>[3x]HHHHHHG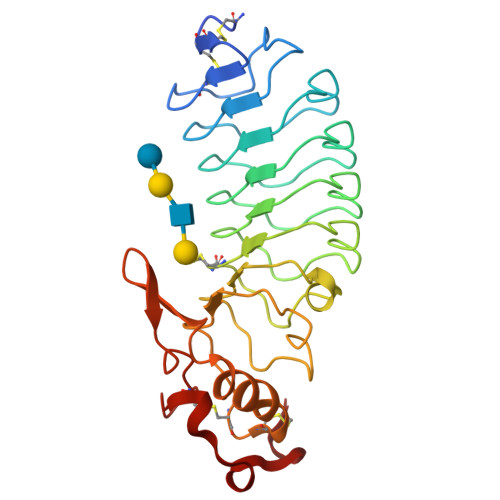GCPSQCSCSGTTVNCKSKSLASVPAGIPTTTRVLYLNDNQITKLEPGVFDRLVNLQTLWLNNNQLTSLPAGLFDSLTQLTILALDSNQLQALPVGVFGRLVDLQQLYLGSNQLSALPSAVFDRLVHLKELLMCCNKLTELPRGIERLTHLTHLALDQNQLKSIPHGAFDRLSSLTHAYLFGNPWDCECRDIMYLRNWVADHTSIVMRWDGKAVNDPDSAKCAGTNTPVRAVTEASTSPSKCP>[2x]MGSDKIHHHHHHMPKVEIAPSEIKIPDNVLKAKLGFGGAEEIPEEFRKTVNRAYEELL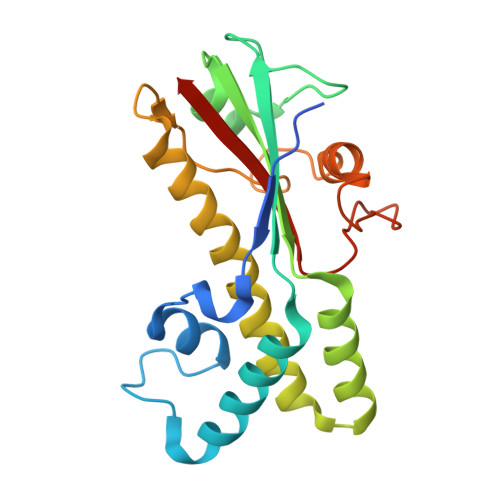DAAKPVVLWRDFEVDGSLSFDDMRLTGELATKHLSGSKIITVFLATLGKKVDEKIEEYFRKGEDLLAFFIDGIASEMVEYALRKVDAELRMKRSNLEGSFRISPGYGDLPLSLNKKIAEIFKEEVDVNVIEDSYVLVPRKTITAFVGWREKNEKQT>[2x]QGLYVGGFVDVVSCPKLEQELYLDPDQVTDYLPVTEP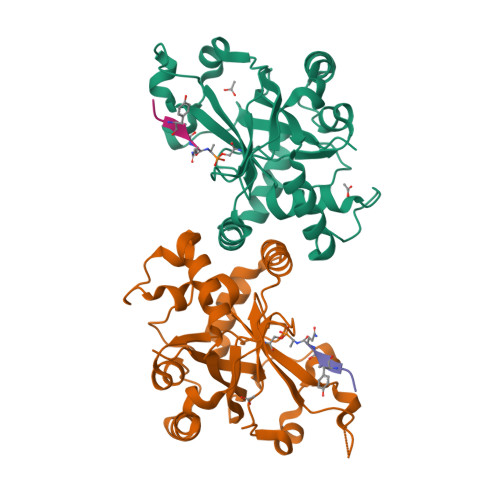LPITIEHLPETEVGWTLGLFQVSHGIFCTGAITSPAFLELASRLADTSHVARAPVKNLPKEPLLEILHTWLPGLSLSSIHPRELSQTPSGPVFQHVSLCALGRRRGTVAVYGHDAEWVVSRFSSVSKSERAHILQHVSSCRLEDLSTPNFVSPLETLMAKAIDAGFIRDRLDLLKTDRGVASILSPVYLKA> MWEQGAPETLQRCLEENQELRDAIRQSNQILRERCEELLHFQA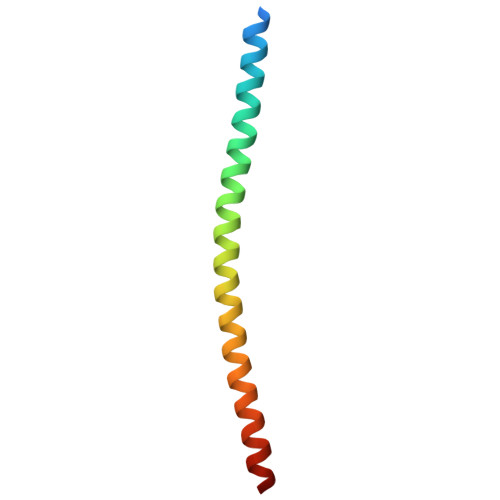SQREEKEFLMCKFQEARKLVERLGLEK> YNRMKLMIVGNTGSGKTTLLQQLMKTKKSDLGMQSATVGIDVKDWPIQIRDKRKRDLVLNVWDFAGREEFYSTHPHFMTQRALYLAVYDLSKGQAEVDAMKPWLFNIKARASSSPVILVGTHLDVSDEKQRKACMSKITKELLNKRGFPAIRDYHFVNATEESDALAKLRKTIINESLNFKIRDQLVVGQLIPD

Leucine-rich repeat kinase 2 (LRRK2) is one of the most commonly mutated genes in familial Parkinson’s disease (PD). The carboxy-terminal half contains LRRK2’s enzymatic domains—both a Roco family GTPase (Ras-of-complex or ROC domain) and a kinase—as well as a scaffolding domain (C-terminal of ROC, or COR) and a WD40 domain. In vitro, the catalytic half of LRRK2 alone can bind to microtubules. Here, we report cryo-EM structures of microtubule-bound filaments formed by LRRK2RCKW.

Unlike WT LRRK2RCKW and LRRK2RCKW-G2019S, LRRK2RCKW-I2020T showed this additional layer line in the absence of MLi-2 as well. Given these observations, we chose the LRRK2RCKW-I2020T filaments that formed in the presence of MLi-2 for our cryo-EM work. The ROC domain points towards and contacts the microtubule. In contrast, our cryo-EM map showed clear density connecting LRRK2RCKW and the microtubule. The fact that microtubules are directional polymers, with ‘+’ (fast-growing) and ‘–’ (slow-growing) ends, means that the ROC domains, which would otherwise be related by a twofold symmetry axis perpendicular to the microtubule, are in different local environments. In agreement with this, their connections to the microtubule became apparent only when LRRK2RCKW monomers were refined individually. The higher resolution of our map, and our ability to process LRRK2RCKW monomers individually, allowed us to circumvent the symmetry mismatch between the LRRK2 filaments and the microtubule, and show that LRRK2RCKW monomers related by (pseudo) twofold symmetry in the filament are indeed not truly symmetric and interact with the microtubule differently. A sequence alignment of LRRK1 and LRRK2 revealed several basic patches in LRRK2’s ROC domain that are not well conserved in LRRK1. These basic patches create a positively charged surface facing the microtubule that is absent in LRRK1. The patches correspond to residues 1356–1359 (KTKK in human LRRK2), 1383–1386 (KRKR in human LRRK2), and 1499–1502 (KLRK in human LRRK2). In our highest resolution maps, in which we refined individual LRRK2RCKW monomers in the filament and their contacts with the microtubule, the strongest density connecting LRRK2RCKW to tubulin involves the 1356–1359 and 1383–1386 basic patches.>MTGAKRKKKSMLWSKMHTPQCEDIIQWCRRRLPILDWAPHYNLKENLLPDTVSGIMLAVQQVTQGLAFAVLSSVHPVFGLYGSLFPAIIYAIFGMGHHVATGTFALTSLISANAVERIVPQNMQNLTTQSNTSVLGLSDFEMQRIHVAAAVSFLGGVIQVAMFVLQLGSATFVVTEPVISAMTTGAATHVVTSQVKYLLGMKMPYISGPLGFFYIYAYVFENIKSVRLEALLLSLLSIVVLVLVKELNEQFKRKIKVVLPVDLVLIIAASFACYCTNMENTYGLEVVGHIPQGIPSPRAPPMNILSAVITEAFGVALVGYVASLALAQGSAKKFKYSIDDNQEFLAHGLSNIVSSFFFCIPSAAAMGRTAGLYSTGAKTQVACLISCIFVLIVIYAIGPLLYWLPMCVLASIIVVGLKGMLIQFRDL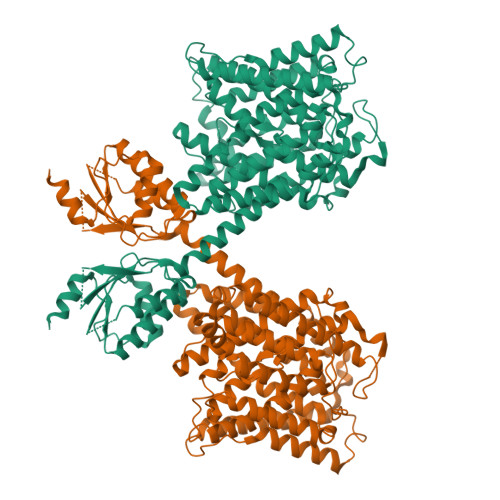KKYWNVDKIDWGIWVSTYVFTICFAANVGLLFGVVCTIAIVIGRFPRAMTVSIKNMKEMEFKVKTEMDSETLQQVKIISINNPLVFLNAKKFYTDLMNMIQKENACNQPLDDISKCEQNTLLNSLSNGNCNEEASQSCPNEKCYLILDCSGFTFFDYSGVSMLVEVYMDCKGRSVDVLLAHCTASLIKAMTYYGNLDSEKPIFFESVSAAISHIHSNKNLSKLSDHSEV[2x]> GAGCAGACCAGA;> CGGCACTCA;> TCTCCG;> TCTGAGTGGGTCTGC

In this work, we exhaustively probe the ability of all 36 immobile HJ sequences to form DNA crystals in two different designed systems. Three separate self-assembling DNA crystal systems are described in this report: the “4 × 5” and “4 × 6” designs (collectively referred to as the 4 × N systems), and a third construct with a “scrambled” sequence variant of the 4 × 6 lattices. Self-assembly was mediated by three constituent oligonucleotides: (S1) containing four sequence repeats of either 5 or 6 bases; (S2) composed of 21 bases containing complementary regions to both (S1); and (S3) which forms the second junction crossover. The HJ serves as the fundamental component at the core of each unit, and the ultimate assembly of the full lattice is facilitated by the complementary 2-base sticky ends that tail each duplex.

Seventeen of the 36 junctions successfully crystallized, a 47% success rate. Unlike the 4 × 5 motif, nearly all of the 4 × 6 junction sequences had a strong preference for crystallization in buffers containing ≥2.0 M salts (e.g., LiCl, Li2SO4, KCl, and NaCl), with the majority preferring slightly basic pH conditions in cacodylic acid. The average cell constants for the P32 crystals were a = b = 68.29 Å c = 55.68 Å. The c-axis, in particular, was ~5 Å shorter, and had a much larger degree of variability (σ = 1.97), than those that crystallized using the 4 × 5 motif. The broad range of the short axis spanned from 52.77 to 60.36 Å, and we posit that the flexible axis lengths could be responsible for rendering a larger number of junctions fatal than the 4 × 5 system. The average junction angles of 54.60° (σ = 1.44) and 58.37° (σ = 2.3) for the P32 and R3 symmetries, respectively, along with their preference for salts or organic solvents, were likely the major contributing factors that yielded the divergent lattices.N-{7-[(1S)-1-methoxyethyl]-2-methyl[1,3]thiazolo[5,4-b]pyridin-6-yl}-N'-[6-(2H-1,2,3-triazol-2-yl)-5-(trifluoromethyl)pyridin-3-yl]urea | 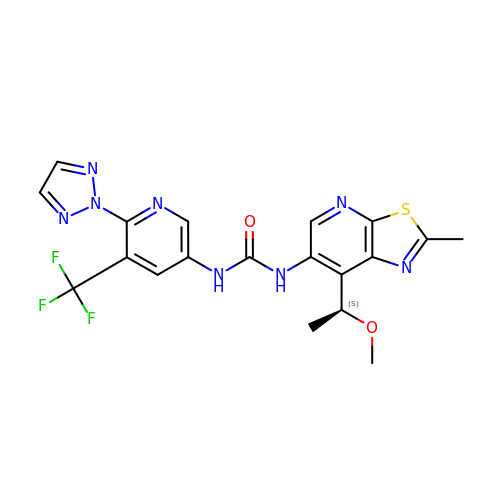C19 H17 F3 N8 O2 S | UVUPDKHEDALPJC-UHFFFAOYSA-N cycloheptyl{4-[(isoquinolin-5-yl)sulfonyl]piperazin-1-yl}methanone | C21 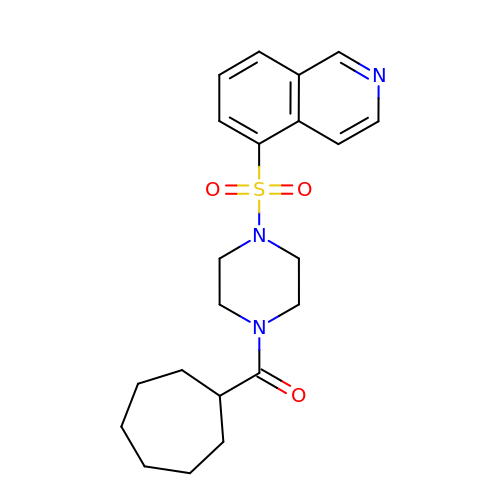H27 N3 O3 S | BNXUOKAWQPMNQC-UHFFFAOYSA-N>AQSRTLLAGIVQQQQQLLDVVKRQQELLRLTVWGTKNLQTRVTAIEKYLKDQAQL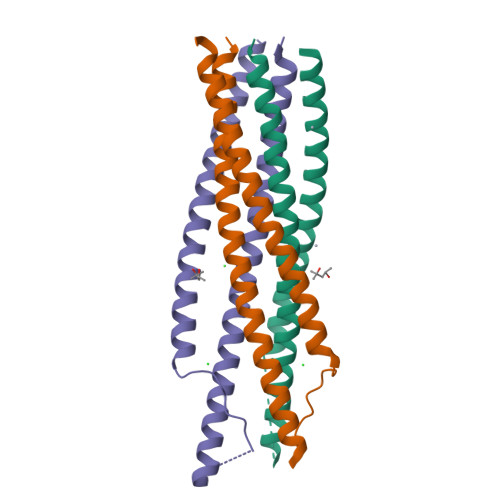NAWGAAFRQVAHTTVPWPNASLTPKWNNETWQEWERKVDFLEENITALLEEAQIQQEKNMYELQKLNS[3x]2-Propen-1-ol | C3 H6 O | 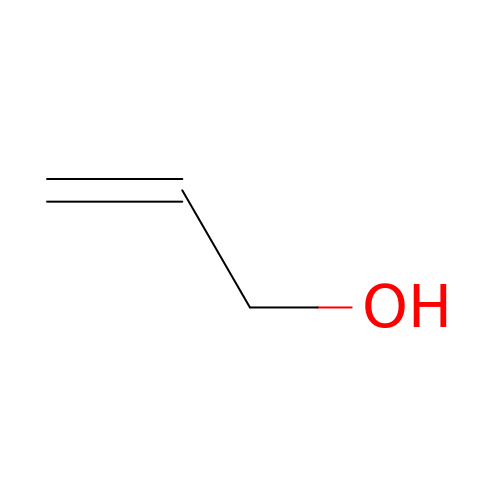XXROGKLTLUQVRX-UHFFFAOYSA-N> MGSSHHHHHHSSGENLYFQSPPPELLEIINEDIAKRTCEEHQLCVVAVLPHILDTGAAGRNSYLEVLLKLADKYKKKMWGWLWTEAGAQSELETALGIGGFGYPAMAAINARKMKFALLKGSFSEQGINEFLRELSFGRGSTAPVGGGA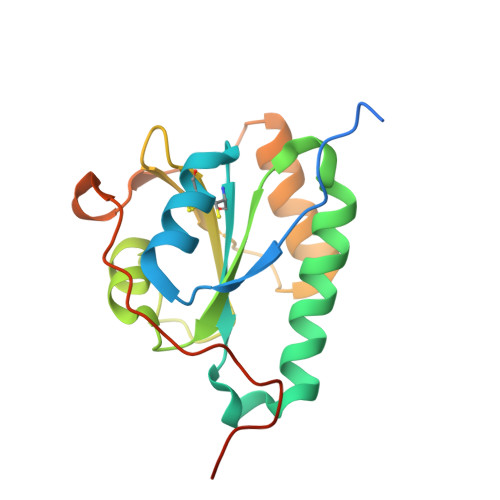FPTIVEREPWDGRDGELPVEDDIDL> ELTPDQATLLHFIMDSYNKQRMPQEITNKILKEAFSAEENFLILTEMATNHVQVLVE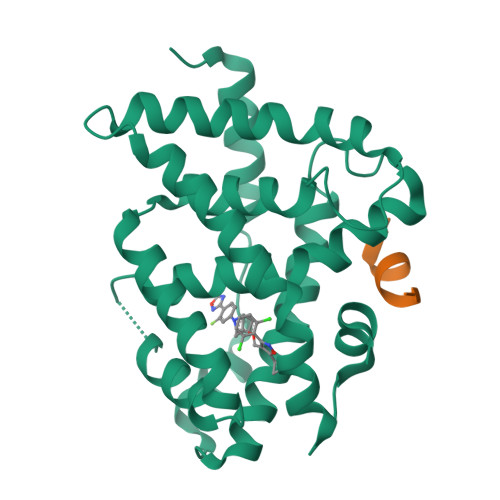FTKKLPGFQTLDHEDQIALLKGSAVEAMFLRSAEIFNKKLPSGHSDLLEARIRNSGISDEYITPMFSFYKSIGELKMTQEEYALLTAIVILSPDRQYIKDREAVEKLQEPLLDVLQKLCKIHQPANPQHFAKLLGRLTELRTFNHHHAEMLMSWRVNDHKFTPLLQEIWDV;> HKILHRLLQDS> MSVVTKSIVNADAEARYLSPGELDRIKNFVSTG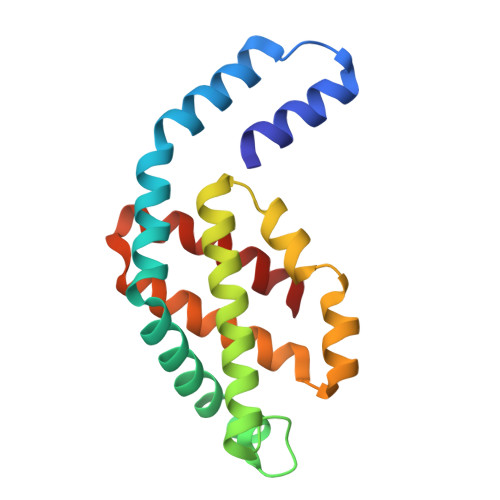ERRLRIAQTLTENRERIVKQAGDQLFQKRPDVVSPGGNAYGEEMTATCLRDLDYYLRLVTYGIVAGDVTPIEEIGLVGVREMYNSLGTPIPAVAEGIRAMKNVACSLLSAEDAAEAGSYFDFVIGAMQ> YGKPGPDGPDGPKGKPGPKG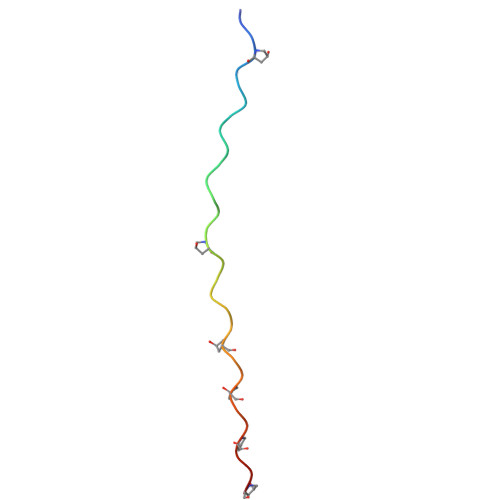KPGKPGKPGKPG> AKCVSYGVSQIKAPALHSQGYTGSNVKVAVIDSGIDSSHPDLNVAGGASFVPSETNPFQDNNSHGTHVAGTVLAVAPSASLYAVKVLGADGSGQYSWIINGIEWAIANNMDVINMSLGGPSGSAALKAAVDKAVASGVVVVAAAGNEGTSGSSSTVGYPGKYPSVIAVGAVDSSNQRASFSSVGPELDVMAPGVSICSTLPGNKYGAKSGTSMAS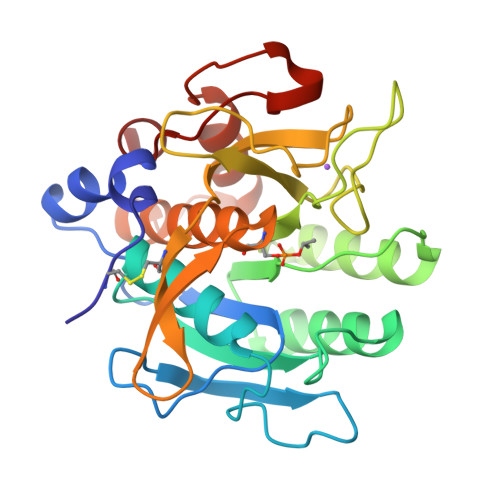PHVAGAAALILSKHPNWTNTQVRSSLENTTTKLGNSFYYGKGLINVQAAAQ> MLLNPTKRERKENYSIDNYYKDVLNTGRSSTPSHPRMPKPHVFHSHQLQPPQLKVLYEKERMWTAKKTGYVPTMDDVKAAYGDISDEEEKKQKLELLKLSVNNSQPLTEEEEKMKADWESEGFTNWNKLEFRKFITVSGKYGR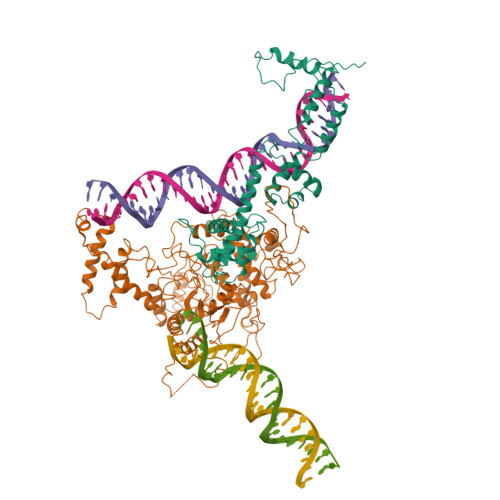NSIQAIARELAPGKTLEEVRAYAKAFWSNIERIEDYEKYLKIIENEEEKIKRVKMQQEALRRKLSEYKNPFFDLKLKHPPSSNNKRTYSEEEDRFILLMLFKYGLDRDDVYELVRDEIRDCPLFELDFYFRSRTPVELARRGNTLLQCLEKEFNAGIVLDDATKDRMKKEDENGKRIREEFADQTANEKENVDGVESKKAKIEDTSNVGTEQLVAEKIPENETTHHHHHHH;> MVAPKPKPAHEQVEPALIPSNWTSVIPLLTSDFKNQYSVISRLKNPNMKPVPYAGDIIKLMAFINKFSSFFHSDLQNLSFQDFEVGLDLYPGDPNGSAAGIVKGPEDTSLLLYPDFMAIKDIVYCQDKMNLLFLSLLDLTFTENFDGKSAKKKGPLTTWENLKSSSKKVFSNPLYRLRLVAREWGYPREWRQQLPSDQDISKPKTALFEQDEQTPVVDPSHPEILTPNIYTWNANEPLPLESNPLYNREMDKNGILALKPMDRVVLLRALTDWCASHSSAIHDEIYKLTHGKKDPVFGIQTQQVPRYTIEGVDNTINQFKKLCSLIQSRYEIRSKKKHFVKQLKEGKKPDLSRKLEILKEIKAELKNAVKSEKDELLFSLYDKWVPLFEGELPDQPLANPFSERLYKLRLQEFFLGRVPHIGDFYMPRLHSYGDSLEMSTFTDLRNLQALLSKFKNNEYNAFTLFENDGQSMSAQFKLFYHDTPSLAHDVARGRNTSGKVYWYELCHDSATLLEFLEFLDYKIVKPQDEKKEGNEKEKEALNNEAHILEQKSTTDNNPSINTNPLPKDAKYNTARKKLQILKEFLSDYYFILRQFEQMKVQFADMKPGKRQLRRIQRQTVNYNT>MIAMIVKGGLAMAISNGHVSFKRPAWLGDSITANNGLATVHYHDILAADWDVERSDNLGISGSTIGSRYDAMAVRYQAIPEDADFIAVFGGVNDYGRDQPLGQYGDCDMTTFYGALMMLLTGLQTNWPTVPKLFISAIHIGSDFGGSFSAVTNGLGYRQSDYEAAIAQMTADYGVPHLSLYRDAGMTFAIPAQA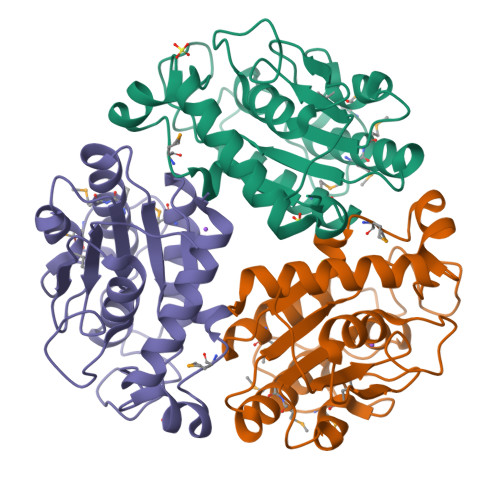AIYSVDTLHPNNAGHRVIARKLQSFLDSHFLEHHHHHH[3x]> TSWSDRLQNAADMPANMDKHALKKYRREAYHRVFVNRSLAMEKIKCFGFNMDYTLAVYKSPEYESLGFELTVERLVSIGYPQELLSFAYDSTFPTRGLVFDTLYGNLLKVDAYGNLLVCAHGFNFIRGPETREQYPNKFIQRDDTERFYILNTLFNLPETYLLACLVDFFTNCPRYTSCETGFKDGDLFMSYRSMFQDVRDAVDWVHYKGSLKEKTVENLEKYVVKDGKLPLLLSWMKEVGKVFLATNSDYKYTDKIMTYLFDFPHGPKPGSSHRPWQSYFDLILVDARKPLFFGEGTVLRQVDTKTGKLKIGTYTGPLQHGIVYSGGSSDTICDLLGAKGKDILYIGDHIFGDILKSKKRQGWRTFLVIPELAQELHVWTDKSSLFEELQSLDIFLAELYKHLDSSSIQRRIKKVTHDMDMCYGMMGSLFRSGSRQTLFASQVMRYADLYAASFINLLYYPFSYL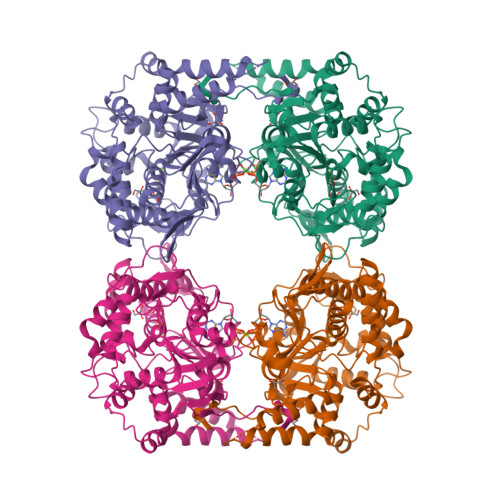FRAAHVLMPHES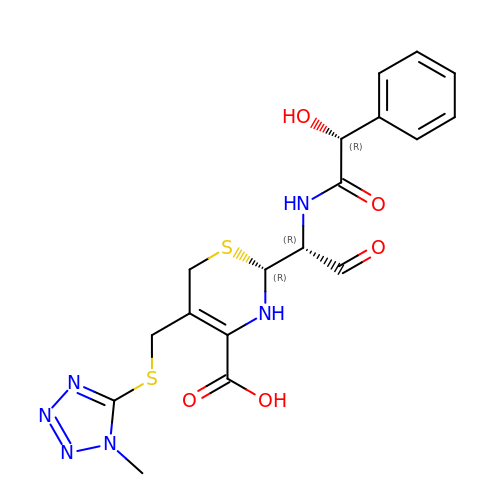(2R)-2-[(1R)-1-{[(2R)-2-hydroxy-2-phenylacetyl]amino}-2-oxoethyl]-5-{[(1-methyl-1H-tetrazol-5-yl)sulfanyl]methyl}-3,6-dihydro-2H-1,3-thiazine-4-carboxylic acid | C18 H20 N6 O5 S2 | CTWPBVTUYYLUGC-XNRPHZJLSA-N> GHMASVNAETVAPEFIVKVRKKLSLTQKEASEIFGGGVNAFSRYEKGNAQPHPSTIKLLRVLDKHPELLNEIR

Our biochemical and structural analysis of the E. coli MqsA antitoxin and the MqsR:MqsA-N complex provide a detailed 3-dimensional structural view of the free antitoxin and the TA complex. These structures combined with our biochemical data unequivocally demonstrate that MqsR, a protein previously shown to be critical for biofilm formation and the most highly upregulated gene in persister cells in E. coli, and MqsA form a novel bacterial TA system. Our data show that, as expected for a TA system, the expression of the MqsR toxin leads to growth arrest, while co-expression with its antitoxin, MqsA, rescues the growth arrest phenotype. In addition, MqsR associates with MqsA to form a tight, non-toxic complex and both MqsA alone and the MqsR:MqsA2:MqsR complex bind and regulate the mqsR promoter. MqsA itself is a two-domain protein with a novel fold that, unlike every other antitoxin, is well-ordered throughout its entire sequence and whose structure does not change upon toxin binding.

MqsA-C, the helix-turn-helix (HTH) domain, is composed of five tightly packed α-helices, which bury a central hydrophobic core. This core is composed of eight residues, including Val69, Val77, Leu83, Phe92, Phe99, Tyr102, Pro109, and Leu117. Of these, all but one (Val69) are perfectly conserved among the MqsA family. Structural similarity searches demonstrated that MqsA-C shows significant homology to the bacteriophage 434 Cro repressor, the P22 C2 repressor and HigA antitoxin, placing it in HTH-XRE family of DNA binding proteins. The MqsA C-terminal domain is necessary and sufficient for binding the mqsR promoter (PmqsR), as incubation of PmqsR with MqsA-C results in a shift in the electrophoretic mobility of the DNA. In contrast, no shift is observed when the DNA is incubated with either MqsA-N alone or the MqsR:MqsA-N complex. These results show that DNA binding is mediated exclusively by MqsA-C. MqsA is the first antitoxin that has been shown experimentally to bind DNA via its C-terminal domain. In MqsA, the HTH-XRE DNA binding helix corresponds to α-helix 4 (α-helix 4 highlighted in green). Moreover, MqsA α-helix 4 is the only stretch of residues that is perfectly conserved among all MqsA proteins. Taken together, these data provide strong evidence that MqsA binds DNA via α-helix 4.> MAIPKIASYPLPVSLPTNKVDWRIDASRAVLLIHDMQEYFVHYFDSQAEPIPSLIKHIQQLKAHAKQAGIPVVYTAQPANQDPAERALLSDFWGPGLSEETAIIAPLAPESGDVQLTKWRYSAFKKSPLLDWLRETGRDQLIITGVYAHIGILSTALDAFMFDIQPFVIGDGVADFSLS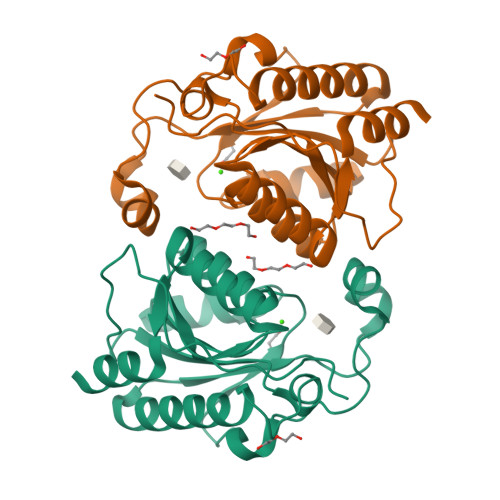DHEFSLRYISGRTGAVKSTQQACLEIAAQHSKLTGLLEHHHHHH> GDPHMACNFQFPEIAYPGKLICPQYGTENKDGEDIIFNYVPGPGTKLIQYEHNGRTLEAITATLVGTVRCEEEKKTDQEEEREGTDQSTEEEKSVDASPNDVTRRTVKNILVSVLPGTEKGRKTNKYANNDFANNLPKEGDIVLTRVTRLSLQRANVEILAVEDKPSPIDSGIGSNGSGIVAAGGG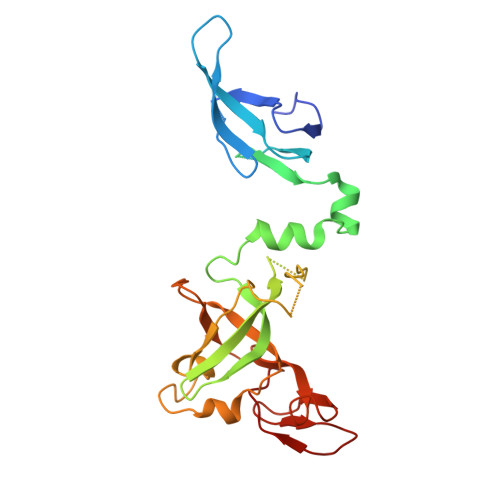SGAATFSVSQASSDLGETFRGIIRSQDVRSTDRDRVKVIECFKPGDIVRAQVLSLGDGTNYYLTTARNDLGVVFARAANGAGGLMYATDWQMMTSPVTGATEKRKCAKPF Two plasmid-encoded dihydrofolate reductase (DHFR) isoforms, DfrA1 and DfrA5, that give rise to high levels of resistance in Gram-negative bacteria were structurally and biochemically characterized to reveal the mechanism of TMP resistance and to support phylogenic groupings for drug development against antibiotic resistant pathogens. TMP is a selective inhibitor of bacterial dihydrofolate reductase (DHFR), which catalyzes the NADPH-dependent reduction of dihydrofolate (DHF) to tetrahydrofolate (THF), a necessary step for the recycling of reduced folate cofactors. Trimethoprim resistance in Enterobacteriaceae occurs almost exclusively through the acquisition of plasmid-associated dfr genes that encode intrinsically insensitive DHFR enzymes. Expectedly, all three enzymes form the stereotypical DHFR fold with an eight-stranded β-sheet, four α-helices (B, C, E, and F) and three catalytic loops (the Met20, F-G, and G-H loops).

The crystal structure of DfrA5:NADPH:TMP, solved to 2.6 Å, reveals major perturbations in the overall ligand binding pose compared to the structures of EcDHFR. Here, the diaminopyrimidine ring of TMP forms interactions with Glu28 (corresponding to Asp27 in EcDHFR); however, the trimethoxyphenyl moiety is oriented horizontally in the pocket, and key van der Waals contacts are lost through the L28Q substitution. Overlay of the EcDHFR:NADPH:TMP and DfrA5:NADPH:TMP structures shows the D27E substitution lays the foundation for the divergent binding orientation of TMP. The additional methylene unit in the side chain of glutamic acid results in a 1.4 Å reorientation of the carboxylate head group, subsequently pulling TMP further into the active site by 1.1 Å. Variations in the GH loop likely enhance the positioning of TMP deeper in the active site of DfrA5 compared to EcDHFR. Although distal to the active site, the GH loop makes critical contacts with helix B (residues 25–35) and is four residues shorter in DfrA5. Downstream effects ultimately cause a 1.9 Å shift in the Cα of Glu28DfrA5 compared to Asp27EcDHFR. Despite co-crystallization and soaking efforts, no density was observed for NADPH in the DfrA1:TMP structure, while in the DfrA5:TMP crystal structure the adenosine and phosphate moiety occupy their expected binding sites. Interestingly, the ribose moiety is oriented away from the active site and the electron density for the nicotinamide is not visible in the crystal structure presumably due to lack of interactions with the protein. Therefore, this somewhat unique conformation of the DfrA5:TMP:NAPDH ternary complex likely prevents favorable interactions between the nicotinamide ring and TMP and contributes to the reduced activity of TMP against this enzyme.

>MKVSLMAAKAKNGVIGCGPHIPWSAKGEQLLFKALTYNQWLLVGRKTFESMGALPNRKYAVVTRSAWTADNDNVIVFPSIEEAMYGLAELTDHVIVSGGGEIYRETLPMASTLHISTIDIEPEGDVFFPNIPNTFEVVFEQHFSSNINYCYQIWQKG[2x]> MHHHHHHMRM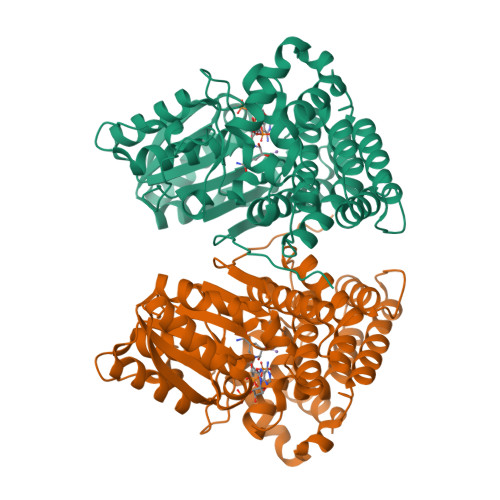EFRHNLPSSDIIFGSGTLEKIGEETKKWGDKAILVTGKSNMKKLGFLADAIDYLESAGVETVHYGEIEPNPTTTVVDEGAEIVLEEGCDVVVALGGGSSMDAAKGIAMVAGHSAEERDISVWDFAPEGDKETKPITEKTLPVIAATSTSGTGSHVTPYAVITNPETKGKPGFGNKHSFPKVSIVDIDILKEMPPRLTAITGYDVFSHVSENLTAKGDHPTADPLAIRAIEYVTEYLLRAVEDGEDIKAREKMAVADTYAGLSNTISGTTLRHAMAHPISGYYPDISHGQALASISVPIMEHNIENGDEKTWERYSRIAVALDASKPVDNTRQAASKAVDGLKNLLRSLDLDKPLSELGVEEEKIPEMTEGAFIYMGGGIEANPVDVSKEDVKEIFRKSL>[2x]MEQVVIVDAIRTPMGRSKGGAFRNVRAEDLSAHLMRSLLARNPSLTAATLDDIYWGCVQQTLEQGFNIARNAALLAEIPHSVPAVTVNRLCGSSMQALHDAARMIMTGDAQVCLVGGVEHMGHVPMSH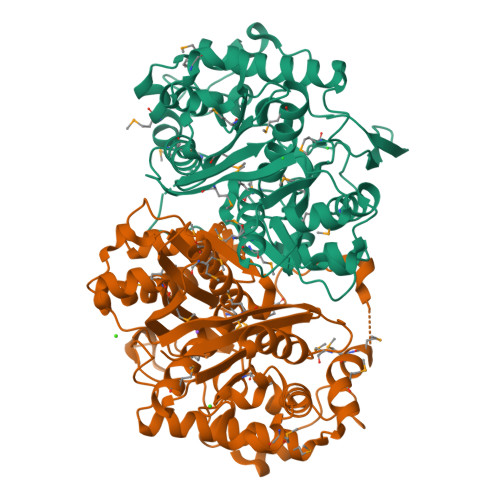GVDFHPGLSRNVAKAAGMMGLTAEMLSRLHGISREMQDQFAARSHARAWAATQSGAFKTEIIPTGGHDADGVLKQFNYDEVIRPETTVEALSTLRPAFDPVSGTVTAGTSSALSDGAAAMLVMSESRARELGLKPRARIRSMAVVGCDPSIMGYGPVPASKLALKKAGLSASDIDVFEMNEAFAAQILPCIKDLGLMEQIDEKINLNGGAIALGHPLGCSGARISTTLINLMERKDAQFGLATMCIGLGQGIATVFERV>MRGSHHHHHHGMASMAVSESQLKKMVSKYKYRDLTVRETVNVITLYKDLKPVLDSYVFNDGSS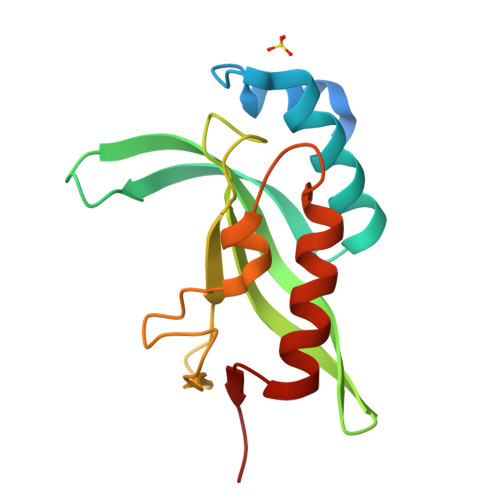RELMNLTGTIPVPYRGNTYNIPICLWLLDTYPYNPPICFVKPTSSMTIKTGKHVDANGKIYLPYLHEWKHPQSDLLGLIQVMIVVFGDEPPVFSRP[2x]ZnT/SLC30 transporters are major players in regulating zinc homeostasis, by harnessing the proton gradient to mobilize the divalent cationic zinc across membranes. ZIPs increase the cytosolic Zn2+ by either importing from the extracellular space or releasing the stored Zn2+ from subcellular compartments, whereas ZnTs remove Zn2+ out of the cytoplasm and maintain physiologically low free Zn2+. ZnT/YiiP mediated Zn2+ transport is mainly powered by proton gradient. Here we determined four high-resolution structures of the plasma-specific hZnT1 and the synaptic vesicle-specific hZnT3.

A global 3.48-Å resolution map was obtained for hZnT1 purified without EDTA treatment, which allows unambiguous modeling of most regions except the intracellular histidine-rich loop (residues 138–240) and the C-terminus (residues 448–507), owing to their intrinsic high mobilities. ZnT1 dimerizes tightly through the intracellular CTDs, the six-helical bundle TMDs, and the extracellular cysteine-rich linker that connects TM5 and TM6 (Figs. 1C and EV2). The extracellular half of TM2 tilt towards the neighboring TM3, which creates a hydrophobic interface mainly through aromatic and aliphatic residues. Openings of both hZnT1 protomers face the extracellular space, revealing a negatively charged chamber at the TMD/ECD nexus. No obvious density was identified in the TMD Zn2+-binding site of either protomer, indicating a Zn2+-unbound OF/OF homodimer captured for ZnT1. Interestingly, the sidechain of His43 on TM2 is not confined in the vicinity of Asp47/His251/Asp255, the highly conserved HD/HD tetrahedral zinc coordination network among ZnT/SLC30 family. Considering that the cytosolic labile Zn2+ concentration ranges from picomolar to nanomolar, while the binding affinity between free Zn2+ and TMD region is measured at the micromolar level with purified ZnT/YiiP proteins, our Zn2+-unbound outward-facing ZnT1 conformation may reflect the post status when zinc ions are expelled out of the translocation passage. In ZnT1, three CTD Zn2+-binding sites were identified at equilateral-triangle positions, in contrast to two closely positioned Zn2+-sites in the YiiP or ZnT8 CTD domains, and none in ZnT7. ZnT1 SCD1 is overlapped with SCD1 sites found in ZnT8 or YiiP proteins, the peripheral SCD2 is composed of residues from both protomers, and the third Zn2+-site (SCD3) is close to the TMD/CTD nexus. Specifically, the Zn2+-chelating network of SIF site is mainly contributed by the intracellular loop residues connecting TM2 and TM3 (IL2-3) in YiiP, or by His137 on IL2-3 and His345 on CTD in ZnT8, while the ZnT1 SCD3 site is composed of CTD residues Glu371 and His373, and the C-terminal extension Cys446 and Cys447.

>[2x]MGCWGRNRGRLLCMLALTFMFMVLEVVVSRVTSSLAMLSDSFHMLSDVLALVVALVAERFARRTHATQKNTFGWIRAEVMGALVNAIFLTGLCFAILLEAIERFIEPHEMQQPLVVLGVGVAGLLVNVLGLCLFHHHSGFSQDSGHGHSHGGHGHGHGLPKGPRVKSTRPGSSDINVAPGEQGPDQEETNTLVANTSNSNGLKLDPADPENPRSGDTVEVQVNGNLVREPDHMELEEDRAGQLNMRGVFLHVLGDALGSVIVVVNALVFYFSWKGCSEGDFCVNPCFPDPCKAFVEIINSTHASVYEAGPCWVLYLDPTLCVVMVCILLYTTYPLLKESALILLQTVPKQIDIRNLIKELRNVEGVEEVHELHVWQLAGSRIIATAHIKCEDPTSYMEVAKTIKDVFHNHGIHATTIQPEFASVGSKSSVVPCELACRTQCALKQCCGTLPQAPSGKDAEKTPAVSISCLELSNNLEKKPRRTKAENIPAVVIEIKNMPNKQPESSLSRLEEELRRRTEGGSSDLEVLFQ3-{7-(trifluoromethyl)-5-[2-(trifluoromethyl)phenyl]-1H-benzimidazol-2-yl}-1-oxa-2-azaspiro[4.5]dec-2-ene 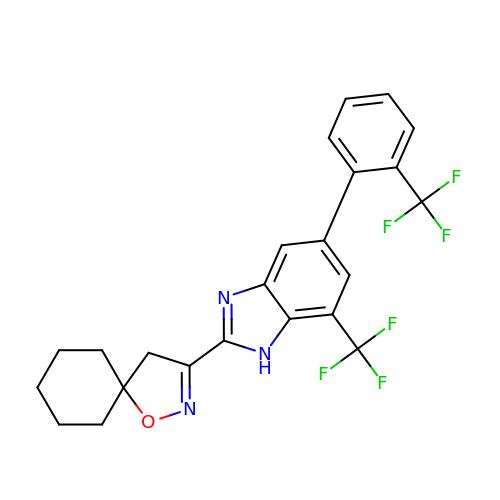| C23 H19 F6 N3 O | VSMFCZZEKTVDHM-UHFFFAOYSA-N>MKWFNTLSHNRWLEQETDRIFDFGKNSVVPTGFGWLGNKGQIKEEMGTHLWITARMLHVYSVAAAMGRPGAYSLVDHGIKAMNGALRDKKYGGWYACVNDEGVVDASKQGYQHFFALLGAASAVTTGHPEARKLLDYTIEIIEKYFWSEEEQMCLESWDEAFSKTEEYRGGNANMHAVEAFLIVYDVTHDKKWLDRAIRVASVIIHDVARNNHYRVNEHFDTQWNPLPDYNKDNPAHRFRAFGGTPGHWIEWGRLMLHIHAALEARCEQP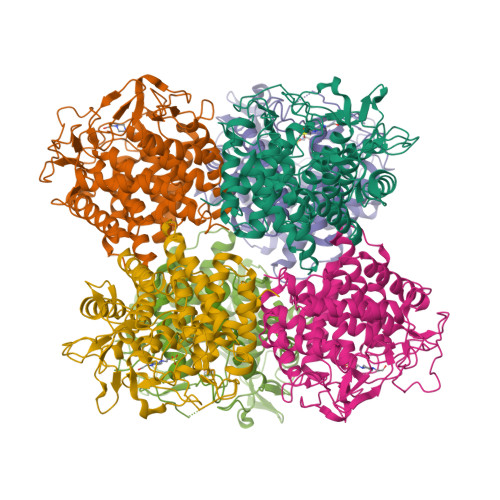PAWLLEDAKGLFNATVRDAWAPDGADGIVYTVDWEGKPVVRERVRWPIVEAMGTAYALYTVTGDRQYETWYQTWWEYCIKYLMDYENGSWWQELDADNKVTTKVWDGKQDIYHLLHCLVIPRIPLAPGMAPAVAAGLLDINAKLEHHHHHH[6x]(2S,3R)-N-[(E)-4-[6,7-bis(chloranyl)-4-oxidanylidene-quinazolin-3-yl]but-2-enyl]-2-(methylamino)-3-oxidanyl-butanamide 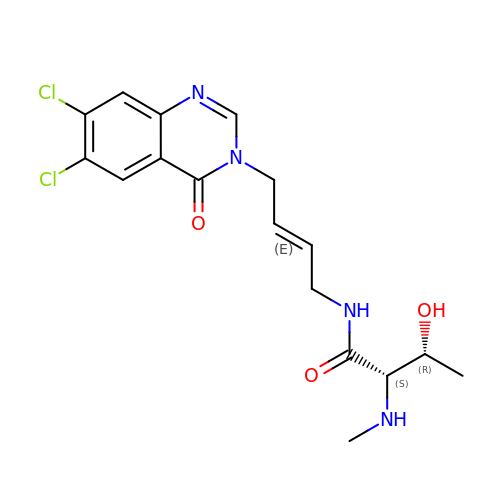| C17 H20 Cl2 N4 O3 | JMUJNICGYNVYJM-BXFHZFJXSA-N DgoR is encoded by the first gene of dgo operon and negatively regulates the whole operon. DgoR was previously predicted to be a FadR family of transcription regulator, and repress the D-galactonate metabolic pathway by binding inverted repeats in the dgo cis-acting element using D-galactonate as a specific effector molecule. As the representative member of GntR superfamily, FadR family is characterized by the presence of a helical domain at the C-terminus (FCD domain). It metabolizes D-galactonate through the enzymes encoded by D-galactonate operon (dgo) and a modified Entner-Doudoroff pathway, where D-galactonate is degraded into D-glyceraldehyde-3-phosphate and pyruvate, and then enter central metabolism.

In our study, we systematically investigated the D-galactonate binding pocket of DgoR using X-ray crystallography, Electrophoretic Mobility Shift Assay (EMSA), and Micro Scale Thermophoresis (MST) assays. Meanwhile, a molecular docking model of the C-terminal domain of E. coli DgoR (EcoDgoR_C) complexed with D-galactonate was established based on the crystal structure of EcoDgoR_C. The key amino acid residues in the binding pocket that are involved in the interactions with D-galactonate were predicted and further validated by site-directed mutational analysis. Moreover, our study shows that some divalent cations (e.g., Zn2+, Mg2+ and Ca2+) are essential for the interaction between DgoR and D-galactonate, but also reveals a unique divalent metal-containing substrate binding pocket, which is the largest one in the GntR superfamily reported so far. The structural information on substrate-enzyme interactions derived from our experimental and docking studies provides a better understanding of the structural and molecular details of effector interactions between sugar acid and the FadR family member.

> MTLNKTDRIVITLGKQIVHGKYVPGSPLPAEAELCEEFATSRNIIREVFRSLMAKRLIEMKRYRGAFVAPRNQWNYLDTDVLQWVLENDYDPRLISAMSEVRNLVEPAIARWAAERATSSDLAQIESALNEMIANNQDREAFNEADIRYHEAVLQSVHNPVLQQLSIAISSLQRAVFERTWMGDEANMPQTLQEHKALFDAIRHQDGDAAEQAALTMIASSTRRLKEIT>MKAVQYTEIGSEPVVVDIPTPTPGPGEILLKVTAAGLCYSDIHVMDMPAAQYAYGLPLTLGHEGVGTVAELGEGVTGFGVGDAVAVYGPWGCGACHACARGRENYCTRAADLGITPPGLGSPGSMAEYMIVDSARHLVPIGDLDPVAAAPLTDAGLTPYHAISRVLPLLGPGSTAVVIGVGGLGHVGIQILRAVSAARVIAVDLDDDRLALAREVGADAAVKSGAGAADAIRELTGGQGATAVFDFVGAQSTIDTAQQVVAVDGHISVVGIHAGAHAKVGFFMIPFGASVVTPFAGTRSELMEVVALARAGRLDIHTETFTL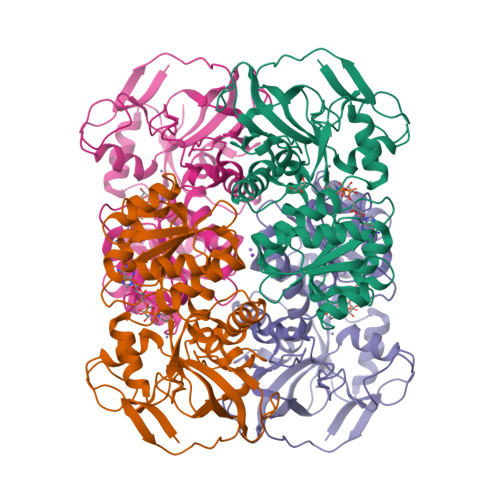DEGPAAYRRLREGSIRGRGVVVPTSHHHHH[4x]>[2x]SMTVKEIFETMDYGPAPESAKEAYAWLAEKGDFGHFIGGAWTAPGDLFATVNPATGQTLAQVSQATQADVDAAVKAARKAQPAWAKDG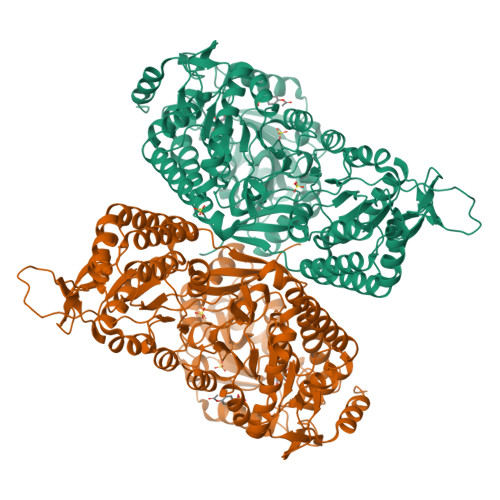AARARVLYALARLLQKHARLFAVLETLDNGKPIREARDIDVPLAQRHFYHHAGYAQLMGTEMPDRAPLGVCGQVIPWNFPLLMLAWKIAPALAMGNTVVLKPAEWTPLTALLFADICGQAGVPAGVVNIVTGDGAVGEMIVTAQVDKVAFTGSTAVGRRIREATAGTGKALSLELGGKGPYVVCDDADIDSAVEGLVDAIWFNQGQVACAGSRLLVQEGIADVFHAKLRARMDSLRIGDPLDKCIDIGAMVHPDQLARVRDMVAANTDGEVYQTAVPAGCYYPPTLISGLAPASPLMQQEIFGPVLVSTTFRTPAEAVEIANNTAYGLAASVWSENVNLALDLAPKLVAGIVWINGTNMMDAAAPFGGVRESGFGREGGWEGLAGYTRPAIATKSPAAVAAYTGDGAADGLDRTAKLYIGGKQTRPDGGYSRAVYGPKGKLLGHASLSNRKDLRNAVEAMNAASGWSRTTGHLRAQILYFIGENLSARADEFANRIKDMTGKDGKAEVAASIDRLFSAAAWADKYDGQVKGVPLRGVALAMKEPVGKIGILCPDAAPLLGLVSLMAPAIAMGNRVTLAASEAFPLAATDFYQVLDTSDVPAGVVNILTGAHADLAEPMARHLDLDAVWGLSGHAQVIEAASAGNLKRSWTGPFDPAHDHTRDILSHATEVKTIWVPYGA> MEGLAGYVYKAASEGKVLTLAALLLNRSESDIRYLLGYVSQQGGQRSTPLIIAARNGHAKVVRLLLEHYRVQTQQTGTVRFDGYVIDGATALWCAAGAGHFEVVKLLVSHGANVNHTTVTNSTPLRAACFDGRLDIVKYLVENNANISIANKYDNTCLMIAAYKGHTDVVRYLLEQRADPNAKAHCGATALHFAAEAGHIDIVKELIKWRAAIVVNGHGMTPLKVAAESCKADVVELLLSHADCDRRSRIEALELLGASFANDRENYDIIKTYHYLYLAMLERFQDGDNILEKEVLPPIHAYGNRTECRNPQELESIRQDRDALHMEGLIVRERILGADNIDVSHPIIYRGAVYADNMEFEQCIKLWLHALHLRQKGNRNTHKDLLRFAQVFSQMIHLNETVKAPDIECVLRCSVLEIEQSMNRVKNISDADVHNAMDNYECNLYTFLYLVCISTKTQCSEEDQCKINKQIYNLIHLDPRTREGFTLLHLAVNSNTPVDDFHTNDVCSFPNALVTKLLLDCGAEVNAVDNEGNSALHIIVQYNRPISDFLTLHSIIISLVEAGAHTDMTNKQNKTPLDKSTTGVSEILLKTQMKMSLKCLAARAVRANDINYQDQIPRTLEEFVGFH;> GGGSGGGSKFADHLHKFHENDNGAAAGDLWQ

We recently discovered that FEM1B, a substrate receptor of Cullin 2-RING ligase (CRL2), recognizes C-degrons containing a C-terminal proline. By solving several cryo-EM structures of CRL2FEM1B bound to different C-degrons, we elucidate the dimeric assembly of the complex. Furthermore, we reveal distinct dimerization states of unmodified and neddylated CRL2FEM1B to uncover the NEDD8-mediated activation mechanism of CRL2FEM1B. Our research also indicates that, FEM1B utilizes a bipartite mechanism to recognize both the C-terminal proline and an upstream aromatic residue within the substrate.

Local refinement was performed on the dimera structure of unCRL2FEM1B-CUX1 to obtain a 3.60 Å resolution structure of the FEM1B-CUX1 subcomplex. The overall architecture of the FEM1B-CUX1 complex exhibits a high degree of structural similarity to that of the FEM1B-CCDC89 complex. Two parts of the CUX1 peptide, −23KFADHLHKFH−14 and −7AAGDLWQ−1, are visible, while the middle 6 residues, −13ENDNGA−8, are invisible. The conformation of the CUX1 C-terminal fragment is slightly different from that of its counterpart in CCDC89. In contrast to the CCDC89 Pro-1 residue, the main chain carbonyl group of CUX1 Gln-1 is hydrogen bonded to the side chain of Ser122 in FEM1B. Trp-2 forms two hydrogen bonds with the side chain of FEM1B Arg126 via its main chain carbonyl group, with its side chain making π-π interactions with the aromatic ring of Tyr84; Leu-3 makes hydrophobic interactions with Tyr163 and Phe193; Asp-4 and Gly-5 make very few interactions with FEM1B residues except that the main chain carbonyl group of Asp-4 is hydrogen bonded to Arg126; and Gly-5 makes hydrophobic interactions with Trp-2 to stabilize the CUX1 conformation. Phe-22 is snugly accommodated into the pocket that was identified earlier as the binding site for CCDC89 His-21. Phe-22 forms hydrophobic interactions with FEM1B Val391 and His502, π-π interactions with Phe501 and Trp367, and a main chain hydrogen bond with Asp356. The favorable π-π interactions suggest that the pocket likely prefers aromatic residues, such as Phe, Tyr, and Trp, over other residues. F-22A decreased the binding affinity by > 170-fold (KDs: >500 vs. 2.8 µM), suggesting that Phe-22 plays a critical role in binding to FEM1B.2-(2-fluorophenyl)-6-methoxy-1,3-benzothiazole | C14 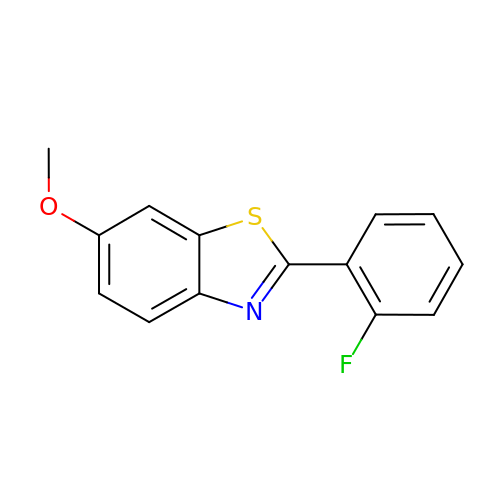H10 F N O S | PPGLEUILAOUYQO-UHFFFAOYSA-N>[2x]MGGHHHHHHGENLYFQGISSETGEMGILWEFDPIINKWIRLSMK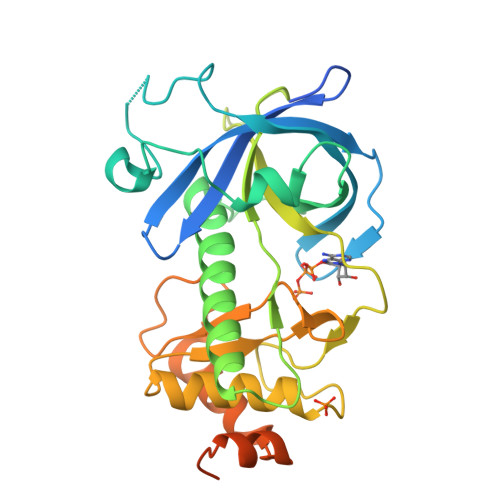LKVERKPFAEGALREAYHTVSLGVGTDENYPLGTTTKLFPPIEMISPISKNNEAMTQLKNGTKFVLKLYKKEAEQQASRELYFEDVKMQMVCRDWGNKFNQKKPPKKIEFLMSWVVELIDRSPSSNGQPILCSIEPLLVGEFKKNNSNYGAVLTNRSTPQAFSHFTYELSNKQMIVVAIQGVDDLYTDPQIHTPDGKGFGLGNLGKAGINKFITTHKCNAVCALLDLDVKLGGVLSGNNKKQLQQGTMVMPDILPELMPSDNT>MKHTVEVMIS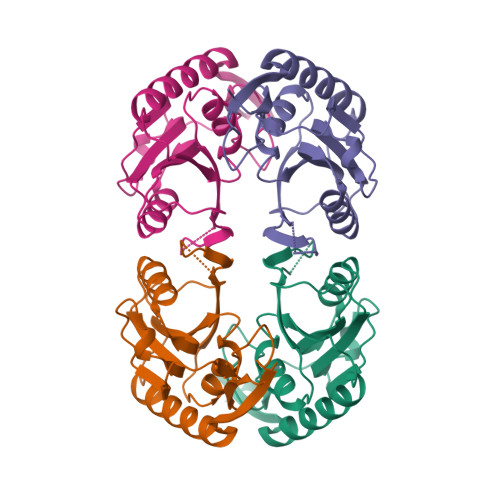EQEVAQRIRELGQQITEHYQGSSDLVLVGLLRGSFVFMADLARQIHLTHQVDFMTASSYGNSMQSSRDVRILKDLDDDIKGKDVLLVEDIIDTGNTLNKVKEILALREPKSIRICTLLDKPTRREVDVEVNWVGFEIPDEFVVGVGIDYAQKYRHLPYIGKVVPLAE[4x]>MEKSNRSLKDLDLNALFIGDKAENGQLYKDLLNKLVDEHLGWRKNYIPSDPNMIGPEDQNSPAFKKTVGHMKTVLDQLSERIRTESVPWHSAGRYWGHMNSETLMPALLAYNYAMLWNGNNVAYESSPATSQMEEEVGQEFARLMGYDYGWGHIVADGSLANLEGLWYARNIKSLPFAMKEVNPELVAGKSDWELLNMPTKEIMDLLENAGSQIDEVKKRSARSGKNLQRLGKWLVPQTKHYSWMKAADIIGIGLDQVVPVPIDSNYRMDIQALESIIRKYAAEKTPILGVVGVAGSTEEGAVDGIDKIVALRQKLQKEGIYFYLHVDAAYGGYARALFLDEDDQFIPYKNLQKVHAENHVFTEDKEYIKPEVYAAYKAFDQAESITIDPHKMGYVPYSAGGIVIQDIRMRDTISYFATYVFEKGADIPALLGAYILEGSKAGATAASVWAAHHTLPLNVTGYGKLEGASIEGAHRYYDFLKNLKFEVAGKRISVHPLISPDFNMVDYVLKEDGND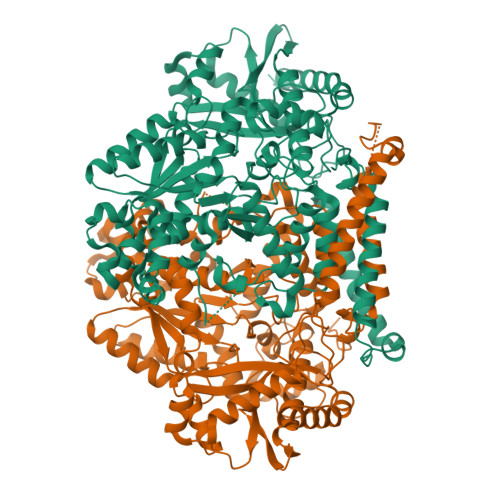DLIEMNRLNHAFYEQASYVKGSLYGKEYIVSHTDFAIPDYGDSPLAFVESLGFSEVEWRHAGKVTIIRASVMTPYMNQRENFDYFAPRIKKAIQADLEKVYASVNQKENVLEHHHHHH[2x]>SELLQRCESLEKKTATFENIVCVLNREVERVAMTAEACSRQHRLDQDKIEALSSKVQQLER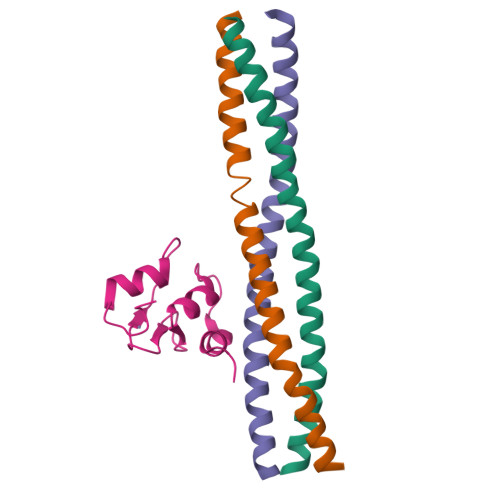SIGLE[3x];> MLSCELYRMSTYSTFPAGVPVSERSLARAGFYYTGVNDKVKCFCCGLMLDNWKRGDSPTEKHKKLYPSCRFVQSL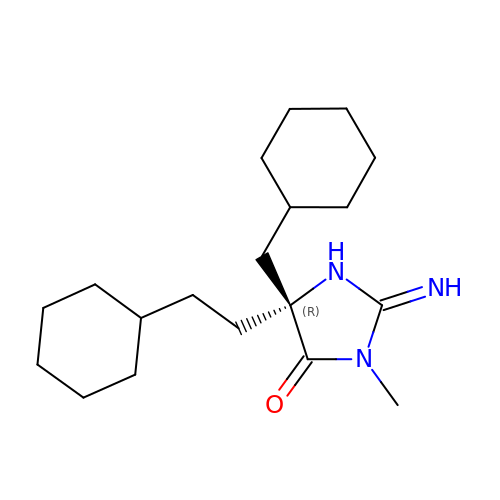(2E,5R)-5-(2-cyclohexylethyl)-5-(cyclohexylmethyl)-2-imino-3-methylimidazolidin-4-one | C19 H33 N3 O | SVQNYPQKWMFQJJ-LJQANCHMSA-N> MGSSHHHHHSSGENLYFQGHMAMEIGEDEWKVCCGSSEFAKQMSTSGPLTSQEAIYTARDIWFNQVNVTDWLEAFSAHPQIGNTPSPSINSDFARRSVSEQSTAFATTSASALQELAEWNVLYKKKFGF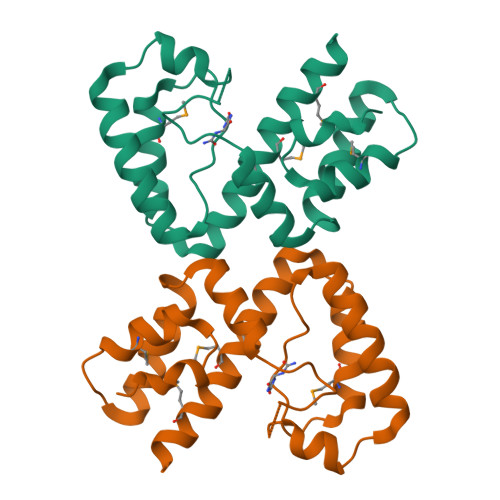IFIICASGRTHAEMLHALKERYENRPIVELEIAAMEQMKITELRMAKLFSDK> MNGAELIIQEINKEAERKIEYILNEARQQAEKIKEEARRNAEAKAEWIIRRAKTQAELEKQRIIANARLEVRRKRLAIQEEIISSVLEEVKRRLETMSEDEYFESVKALLKEAIKELNEKKVRVMSNEKTLGLIA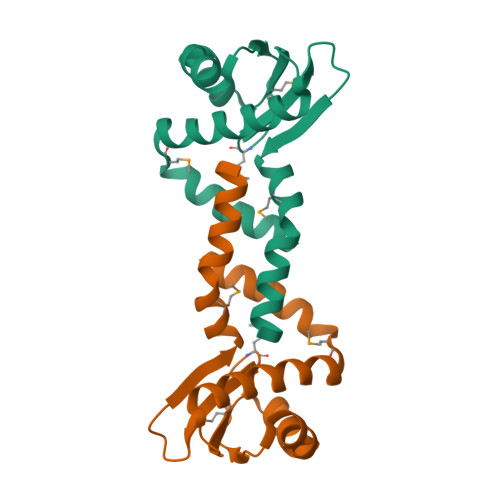SRIEEIKSELGDVSIELGETVDTMGGVIVETEDGRIRIDNTFEARMERFEGEIRSTIAKVLFG> SDILGMLK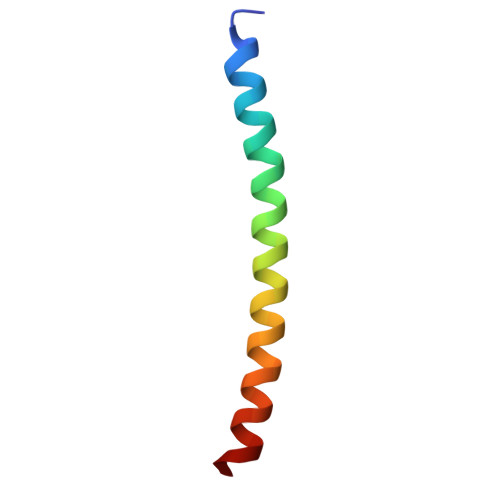SLHQLQVENRRLEEQIKNLTAKKERLQLLNAQLSV>[3x]ALGSNSSSQPNRVARMPVDRNAPYYNMNHKHRGMAIIFNHEHFDIHSLKSRTGTNVDSDNLSKVLKTLGFKVTVFPNLKSEEINKFIQQTAEMDHSDADCLLVAVLTHGELGMLYAKDTHYKPD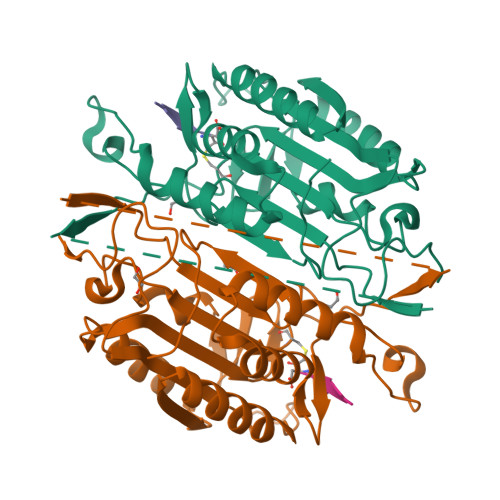NLWYYFTADKCPTLAGKPKLFFIQACQGDRLDGGITLSRTETDGSPSTSYRIPVHADFLIAFSTVPGYFSWRNTTRGSWFMQALCEELRYAGTERDILTLLTFVCQKVALDFESNAPDSAMMHQQKQVPCITSMLTRLLVFGKKQSHL> MNGIYIWKIGNFGMHLKCQEEEKPVVIHSPGFYTGKPGYKLCMRLHLQLPTAQRCANYISLFVHTMQGEYDSHLPWPFQGTIRLTILDQSEAPVRQNH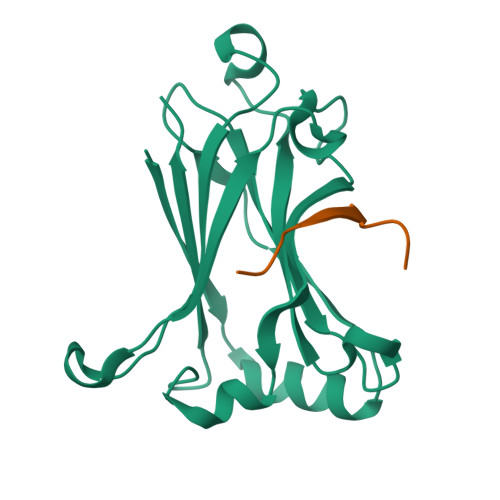EEIMDAKPELLAFQRPTIPRNPKGFGYVTFMHLEALRQRTFIKDDTLLVRCEVSTLEHHHHHH;> SSQSQSPTEDDENES> MALTKVKLLAYQDKRFENKLGEFELPINPEQFSQSFKVEYNREQA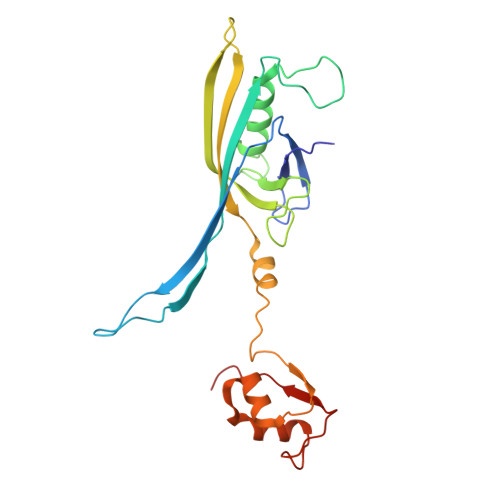QGSQRNDPEFKFTKPEELKLDFTFDGTGVVPVNNGKPGEFHQDVADQVRVFLDLVYSMNSETHKPNFLRLIWGDFSFGEKNGFDCLLTDLQINYTLFDQTGKPLRAKLSTTFTSYVEQNRRVREEGKQSPDVTHQRKVKAGDTLPLMTHRIYGDPAYYLQIAKVNGLINFRKLATNTDLRFPPLEKTQS>[4x]GMNQRDVILDCEKKLLTAIQNNDVESLEVLLHDDLLFIIPSGETVTKETDIAAYSSGKIALRAVVPSDYIIRIIH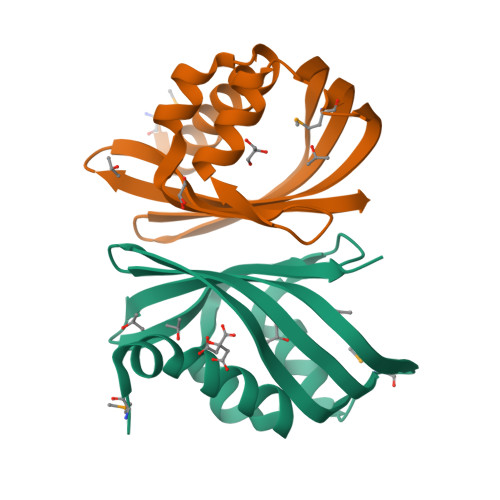DTVVVSVNIEIKGEYMEHTLDNTFRYLRVWKLFDGNWKVIAGSCTAIG> GPLGSAAQGTVRKAGALAVKNFLVHKKNKKVESATRRKWKHYWVSLKGCTLFFYET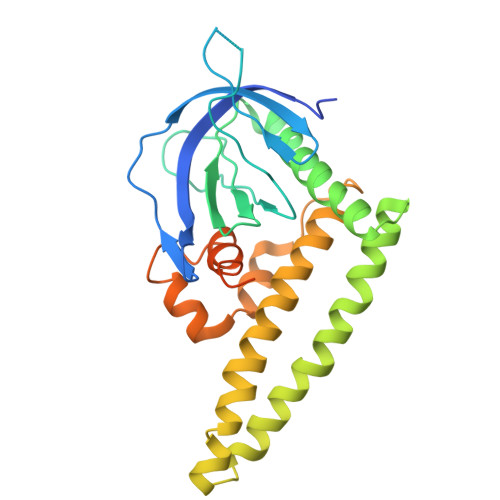DGRSGIDHNSVPKHAVWVENSIVQAVPEHPKKDFVFCLSNSLGDAFLFQTTSQTELENWITAIHSACAAAVARHHHKEDTLRLLKSEIKKLEQKIDMDEKMKKMGEMQLSSVTDSKKKKTILDQIFVWEQNLEQFQMDLFRFRCYLASLQGGELPNPKRLLAFASRPTKVAMGRLGIFSVSSFHALVAARTGEIGVRRRTQAMSRSASKRRSRFSSLWGLDTT> MNLLIDNWIPVRPRNGGKVQIINLQSLYCSRDQWRLSLPRDDMELAALALLVCIGQIIAPAKDDVEFRHRIMNPLTEDEFQQLIAPWIDMFYLNHAEHPFMQTKGVKANDVTPMEKLLAGVSGATNCAFVNQPGQGEALCGGCTAIALFNQANQAPGFGGGFKSGLRGGTPVTTFVRGIDLRSTVLLNVLTLPRLQKQFPNESHTENQPTWIKPIKSNESIPASSIGFVRGLFWQPAHIELCDPIGIGKCSCCGQESNLRYTGFLKEKFTFTVNGLWPHPHSPCLVTVKKGEVEEKFLAFTTSAPSWTQISRVVVDKIIQNENGNRVAAVVNQFRNIAPQ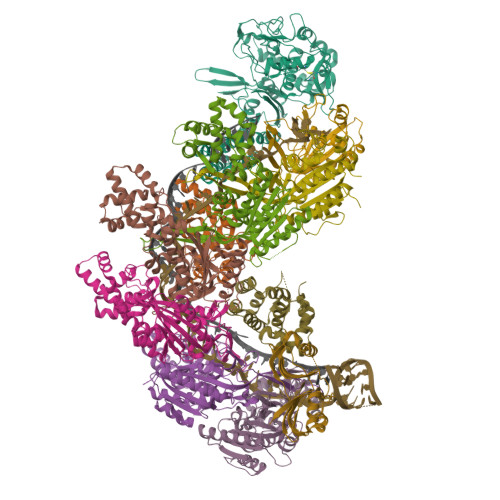SPLELIMGGYRNNQASILERRHDVLMFNQGWQQYGNVINEIVTVGLGYKTALRKALYTFAEGFKNKDFKGAGVSVHETAERHFYRQSELLIPDVLANVNFSQADEVIADLRDKLHQLCEMLFNQSVAPYAHHPKLISTLALARATLYKHLRELKPQGGPSNG;>MADEIDAMALYRAWQQLDNGSCAQIRRVSEPDELRDIPAFYRLVQPFGWENPRHQQALLRMVFCLSAGKNVIRHQDKKSEQTTGISLGRALANSGRINERRIFQLIRADRTADMVQLRRLLTHAEPVLDWPLMARMLTWWGKRERQQLLEDFVLTTNKNA[2x];>MSNFINIHVLISHSPSCLNRDDMNMQKDAIFGGKRRVRISSQSLKRAMRKSGYYAQNIGESSLRTIHLAQLRDVLRQKLGERFDQKIIDKTLALLSGKSVDEAEKISADAVTPWVVGEIAWFCEQVAKAEADNLDDKKLLKVLKEDIAAIRVNLQQGVDIALSGRMATSGMMTELGKVDGAMSIAHAITTHQVDSDIDWFTAVDDLQEQGSAHLGTQEFSSGVFYRYANINLAQLQENLGGASREQALEIATHVVHMLATEVPGAKQRTYAAFNPADMVMVNFSDMPLSMANAFEKAVKAKDGFLQPSIQAFNQYWDRVANGYGLNGAAAQFSLSDVDPITAQVKQMPTLEQLKSWVRNNGEA[6x];> MRSYLILRLAGPMQAWGQPTFEGTRPTGRFPTRSGLLGLLGACLGIQRDDTSSLQALSESVQFAVRCDELILDDRRVSVTGLRDYHTVLGAREDYRGLKSHETIQTWREYLCDASFTVALWLTPHATMVISELEKAVLKPRYTPYLGRRSCPLTHPLFLGTCQASDPQKALLNYEPVGGDIYSEESVTGHHLKFTARDEPMITLPRQFASREWYVIKGGMDVSQ;> MYLSKVIIARAWSRDLYQLHQGLWHLFPNRPDAARDFLFHVEKRNTPEGCHVLLQSAQMPVSTAVATVIKTKQVEFQLQVGVPLYFRLRANPIKTILDNQKRLDSKGNIKRCRVPLIKEAEQIAWLQRKLGNAARVEDVHPISERPQYFSGDGKSGKIQTVCFEGVLTINDAPALIDLVQQGIGPAKSMGCGLLSLAPL>LGQEKERFQVLPGRDKMLYVAAQNERDTLWARQVLARGDYDKNARVINENEENKRISIWLDTYYPQLAYYRIHFDEPRKPVFWLSRQRNTMSKKELEVLSQKLRALMPYADSVNITLMDDVTAAGQAEAGLKQQALPYSRRNHKGGVTFVIQGALDDVEILRARQFVDSY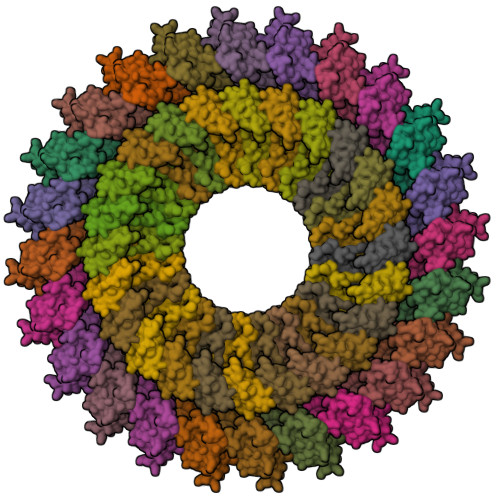YRTWGGRYVQFAIELK[24x];>KDLLKGLDQEQANEVIAVLQMHNIEANKIDSGKLGYSITVAEPDFTAAVYWIKTYQLPPRPRVEIAQMFPADSLVSSPRAEKARLYSAIEQRLEQSLQTMEGVLSARVHISYDIDAGENGRPPKPVHLSALAVYERGSPLAHQISDIKRFLKNSFADVDYDNISVVLSER[24x]The OXA-48 carbapenemase is widely disseminated in Enterobacterales, necessitating new treatments for producer strains. OXA-48 is a class D SBL that uses a nucleophilic serine (Ser70) to hydrolyse β-lactams, with a proximal post-translationally carbamylated lysine (Lys73) proposed to act as the general base for both the acylation and deacylation steps of the reaction. Diazabicyclooctane (DBO) inhibitors, including avibactam and nacubactam, act on a wide range of enzymes to overcome β-lactamase-mediated resistance. Here we describe investigations on how avibactam and nacubactam inhibit OXA-48 and two variants, OXA-163 and OXA-405, with deletions in the β5–β6 loop neighbouring the active site that modify activity towards different β-lactam classes.

Nacubactam is distinguished from avibactam by an extended C2 substituent bearing a 1-aminoethoxy group. Both OXA-163 and OXA-405 have four amino acid deletions within the β5–β6 loop, including of residue Arg214. OXA-163 also has a single amino acid substitution (Ser212Asp) adjacent to the deleted region. Crystal structures were obtained for OXA-163 and OXA-405, as uncomplexed enzymes and in the nacubactam- and avibactam-bound forms. Both OXA-163 and OXA-405 assemble as homodimers in the asymmetric unit. Consistent with their high overall sequence identities, they adopt very similar overall folds and active site arrangements compared to OXA-48. The exception is the Ser70 nucleophile, which is in dual conformations in one of the two chains in the crystallographic dimers of uncomplexed OXA-163 and OXA-405. The respective protein backbones only differ at the β5–β6 loop, which is truncated in the cases of OXA-163 and OXA-405, compared to OXA-48.

>[2x]GPKEWQENKSWNAHFTEHKSQGVVVLWNENKQQGFTNNLKRANQAFLPASTFKIPNSLIALDLGVVKDEHQVFKWDGQTRDIATWNRDHNLITAMKYSVVPVYQEFARQIGEARMSKMLHAFDYGNEDISGNVDSFWLDGGIRISATEQISFLRKLYHNKLHVSERSQRIVKQAMLTEANGDYIIRAKTGYDTKIGWWVGWVELDDNVWFFAMNMDMPTSDGLGLRQAITKEVLKQEKIIP> GSPEKILAQIIQEHREGLDWQEAATRASLSLEETRKLLQSMAAAGQVTLLRVENDLYAISTERYQAWWQAVTRALEEFHSRYPLRPGLAREELRSRYFSRLPARVYQALLEEWSREGRLQLAANTVALAGFT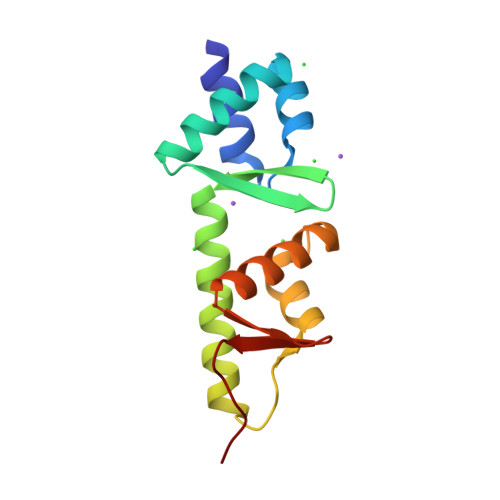PSF>MADPAECSIKVMCRFRPLNEAEILRGDKFIPKFKGEETVVIGQGKPYVFDRVLPPNTTQEQVYNACAKQIVKDVLEGYNGTIFAYGQTSSGKTHTMEGKLHDPQLMGIIPRIAHDIFDHIYSMDENLEF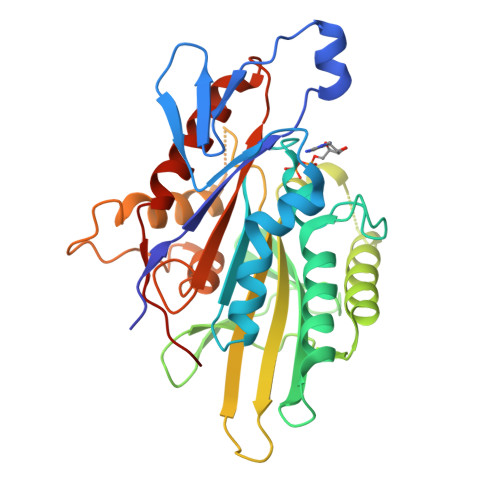HIKVSYFEIYLDKIRDLLDVSKTNLAVHEDKNRVPYVKGCTERFVSSPEEVMDVIDEGKANRHVAVTNMNEHSSRSHSIFLINIKQENVETEKKLSGKLYLVDLAGSEKVSKTGAEGAVLDEAKNINKSLSALGNVISALAEGTKTHVPYRDSKMTRILQDSLGGNCRTTIVICCSPSVFNEAETKSTLMFGQRAKTIKNTVSVNHHHHHHH[2x]Bemnifosbuvir (AT-527) and AT-752 are guanosine analogues currently in clinical trials against several RNA viruses. Here, we show that these drugs require a minimal set of 5 cellular enzymes for activation to their common 5′-triphosphate AT-9010, with an obligate order of reactions. Crystal structures of human histidine triad nucleotide binding protein 1, adenosine deaminase-like protein 1, guanylate kinase 1, and nucleoside diphosphate kinase at 2.09, 2.44, 1.76, and 1.9 Å resolution, respectively, with cognate precursors of AT-9010 illuminate the activation pathway from the orally available bemnifosbuvir to AT-9010, pointing to key drug–protein contacts along the activation pathway.

GUK1 is a nucleoside monophosphate kinase able to transfer a phosphate group from ATP to a guanosine 5′-monophosphate, yielding GDP and ADP. Expectedly, GUK1 is able to phosphorylate GMP into GDP, but also AT-8001 into AT-8500. GUK1 exhibits the highest turnover in the activation chain, but the 2′-C-methyl, 2′-F modification slows it down approximately 200-fold. GUK1 was crystallized and its structure solved at 1.76 Å resolution in complex with AT-8001. Two β-sheets and 8 α-helices, the last 2 separated by a π-helix, define 3 structurally and functionally distinct subdomains: the core, the NMP-binding site, and the lid. The structure presented here is an open conformation, with the AT-8001 substrate binding through extensive contact with both the phosphate moiety and the nucleobase. Thus, on the one hand, Tyr 81, Tyr 53, and Arg 41 share hydrogen bonding with the oxygen of the phosphate, while Arg 44 makes a contact through a water molecule. On the other hand, Glu 72 and Ser 37 engage hydrogen bonds with the base, while Tyr 53 contributes to positioning the base through π-stacking. The protein structurally checks the substrate by contacting both the purine base and the presence of a monophosphate, with no significant check on the ribose at this stage.

>[2x]MSGPRPVVLSGPSGAGKSTLLKRLLQEHSGIFGFSVSHTTRNPRPGEENGKDYYFVTREVMQRDIAAGDFIEHAEFSGNLYGTSKVAVQAVQAMNRICVLDVDLQGVRNIKATDLRPIYISVQPPSLHVLEQRLRQRNTETEESLVKRLAAAQADMESSKEPGLFDVVIINDSLDQAYAELKEALSEEIKKAQRTGA> EDICFIAGIGDTNGYGWGIAKELSKRNVKIIFGIWPPVYNIFMKNYKNGKFDNDMIIDKDKKMNILDMLPFDASFDTANDIDEETKNNKRYNMLQNYTIEDVANLIHQKYGKINMLVHSLANAKEVQKDLLNTSRKGYLDALSKSSYSLISLCKYFVNIMKPQSSIISLTYHASQKVVPGYGGGMSSAKAALESDTRVLAYHLGR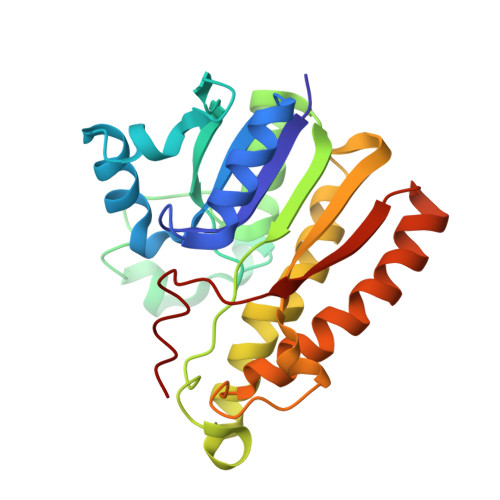NYNIRINTISAGPLKSRAATAINK> METSDIQIFYQEDPECQNLSENSCPPSEVSDTNLYSPFKPRNYQLELALPAMKGKNTIICAPTGCGKTFVSLLICEHHLKKFPQGQKGKVVFFANQIPVYEQQKSVFSKYFERHGYRVTGISGATAENVPVEQIVENNDIIILTPQILVNNLKKGTIPSLSIFTLMIFDECHNTSKQHPYNMIMFNYLDQKLGGSSGPLPQVIGLTASVGVGDAKNTDEALDYICKLCASLDASVIATVKHNLEELEQVVYKPQKFFRKVESRISDKFKYIIAQLMRDTESLAKRICKDLENLSQIQNREFGTQKYEQWIVTVQKACMVFQMPDKDEESRICKALFLYTSHLRKYNDALIISEHARMKDALDYLKDFFSNVRAAGFDEIEQDLTQRFEEKLQELESVSRDPSNENPKLEDLCFILQEEYHLNPETITILFVKTRALVDALKNWIEGNPKLSFLKPGILTGRGKTNQNTGMTLPAQKCILDAFKASGDHNILIATSVADEGIDIAQCNLVILYEYVGNVIKMIQTRGRGRARGSKCFLLTSNAGVIEKEQINMYKEKMMNDSILRLQTWDEAVFREKILHIQTHEKFIRDSQEKPKPVPDKENKKLLCRKCKALACYTADVRVIEECHYTVLGDAFKECFVSRPHPKPKQFSSFEKRAKIFCARQNCSHDWGIHVKYKTFEIPVIKIESFVVEDIATG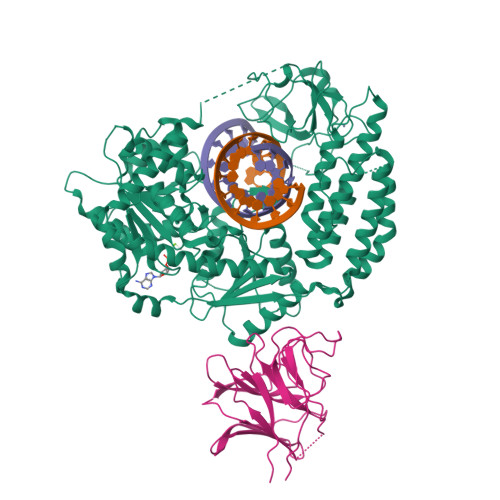VQTLYSKWKDFHFEKIPFDPAEMSK;> RRASRFAQWAIHPTFNLKSLSCSLEVSKDSRTVTVSHRPQPYRWSCERFSTSQVLCSQALSSGKHYWEVDTRNCSHWAVGVASWEMSRDQVLGRTMDSCCVEWKGTSQLSAWHMVKETVLGSDRPGVVGIWLNLEEGKLAFYSVDNQEKLLYECTISASSPLYPAFWLYGLHPGNYLIIKQVKV>MDFSRNLYDIGEQLDSEDLASLKFLSLDYIPQRKQEPIKDALMLFQRLQEKRMLEESNLSFLKELLFRINRLDLLITYLNTRKEEMERELQTPGRAQISAYRVMLYQISEEVSRSELRSFKGGLQEEISKCKLDDDMNLLDIFIEMEKRVILGEGKLDILKRVCAQINKSLLKIINDYEEFSKER[5x];>MSAEVIGQVEEALDTDEKEMLLFLCRDVAIDVVPPNVRDLLDILRERGKLSVGDLAELLYRVRRFDLLKRILKMDRKAVETHLLRNPHLVSDYRVLMAEIGEDLDKSDVSSLIFLMKDYMGRGKISKEKSFLDLVVELEKLNLVAPDQLDLLEKCLKNIHRIDLKTKIQKYKQSVQGAGTS[4x];> MDPFLVLLGSVSSSLSSSELTELKFLCLGRVGKRKLERVQSGLDLFSMLLEQNDLEPGHTELLRELLASLRRHDLLRRVDDFEAGAAAGAAPGEEDLCAAFNVICDNVGKDWRRLARQLKVSDTKIDSIEDRYPRNLTERVR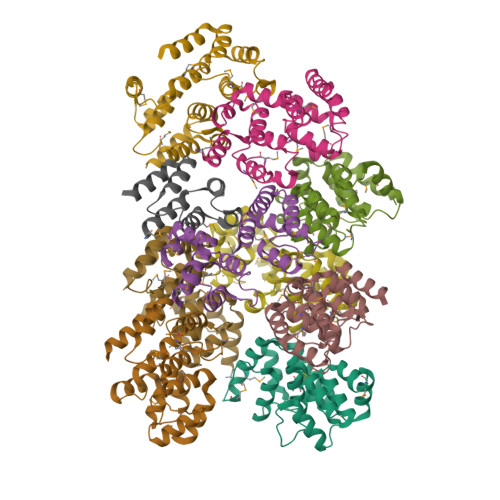ESLRIWKNTEKENATVAHLVGALRSCQMNLVADLVQEVQQARDLQNRSGAMSPMSWNSDASTSEASLEHHHHHH> CAAGAGCCTGATCGGACAAGCGACGCAAGCA;> GAGCAGCCTGTACGGACATCAGTCTCTGCTACTACGTCAGCA;> AACCTACCTGGCAGGACGACTCACTATGCTA;> TGTGCTTGCGTCGCTTGTGGCTGC;> TTTAGCATAGTGAGTCGTGGCTCT;> TCTGCTGACGTAGTAGCAGAGACTGATGTGGTAGG;> TACACCGATCAC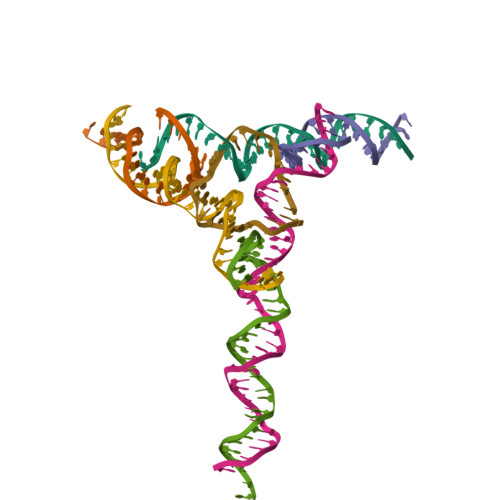CTGCCACCG>GMTTPPARTAKQRIQDTLNRLELDVDAWVSTAGADGGAPYLVPLSYLWDGETFLVATPAASPTGRNLSETGRVRLGIGPTRDLVLVEGTALPLEPAGLPDGVGDTFAEKTGF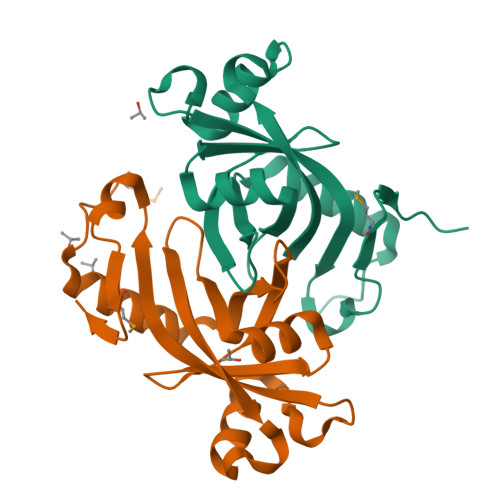DPRRLTTSYLYFRISPRRVQAWREANELSGRELMRDGEWLVTD[2x]>[2x]MRIEVVNVSHIFHRGTPLEKKALENVSLVINEGECLLVAGNTGSGKSTLLQIVAGLIEPTSGDVLYDGERKKGYEIRRNIGIAFQYPEDQFFAERVFDEVAFAVKNFYPDRDPVPLVKKAMEFVGLDFDSFKDRVPFFLS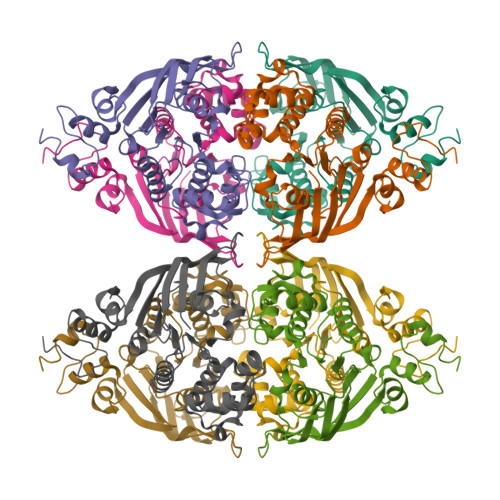GGEKRRVAIASVIVHEPDILILDEPLVGLDREGKTDLLRIVEKWKTLGKTVILISHDIETVINHVDRVVVLEKGKKVFDGTRMEFLEKYDPRFFTSKMLVMRRLVLKGEDPFSMSDDELLERVCNS> GAMEFERAKAAVESDTEFWDKMQAEWEEMARRNWISENQEAQNQVTVSASEKGYYFHTENPFKDWPGAFEEGLKRLKEGDLPV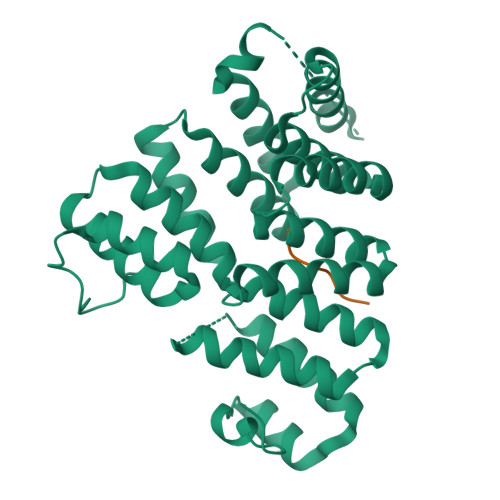TILFMEAAILQDPGDAEAWQFLGITQAENENEQAAIVALQRCLELQPNNLKALMALAVSYTNTSHQQDACEALKNWIKQNPKYKYLVKNKKGSPGLTRRMSKSPVDSSVLEGVKELYLEAAHQNGDMIDPDLQTGLGVLFHLSGEFNRAIDAFNAALTVRPEDYSLWNRLGATLANGDRSEEAVEAYTRALEIQPGFIRSRYNLGISCINLGAYREAVSNFLTALSLQRKSRNQQQVPHPAISGNIWAALRIALSLMDQPELFQAANLGDLDVLLRAFNLDP;> SRLSSNL>[4x]MTSEKIASLRQEIETYLNTGLLPFWITRTVDKENGGFLTHFDQFGNDSGEDEKSLIAQSRSVFTYSSAHRAG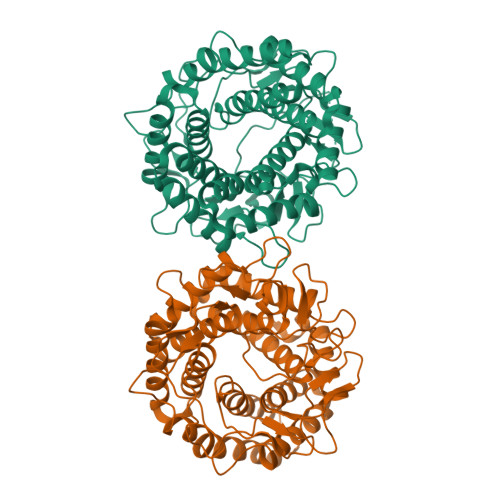YGGGVLAEMARHGVDYLINNMWDNEHGGFYWMTNRKGEVTIDQKIVYGLSFCIYSLSEYTLATGDPRGREYAEKTFDLLQKYAVDTHYGGYFEMFNRDWTLKGPGAAGGDRKTLDVHMHLMEAYTTLYECTGQEIHRRKLLETIELLVNKVMHPEYGTGIPQFWADWSVAPQIKFDIVWGWDRFNPDGLKSAAEDNTSYGHNSEFAWLLMHALDILGLPYDTYREQITKSYTHAVENGVDWEFGGVYVEGSHAGQVYDKEKEFWQQAEMLIGMLDAYRFLKDEKYLQAYENIHRFVFDKMINHSLGEWWPLMTREGVPIWKHMSHSWKINYHDVRSMIQSIVRLDKIAKGV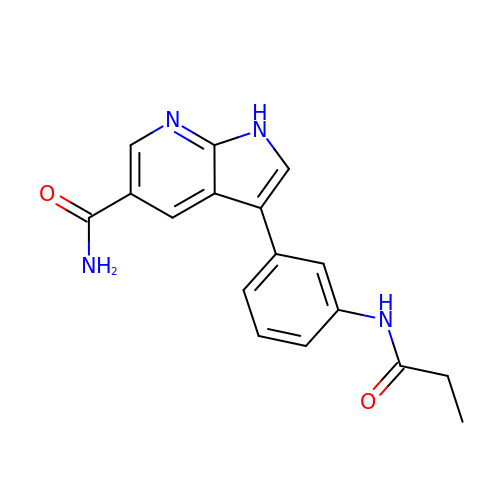3-[3-(propanoylamino)phenyl]-1~{H}-pyrrolo[2,3-b]pyridine-5-carboxamide | C17 H16 N4 O2 | GDAPVGRIYBMGOP-UHFFFAOYSA-N> SGVDDDMACHKIPVEADFLYAYSTAPGYYSWRNSKDGSWFIQSLCAMLKQYADKLEFM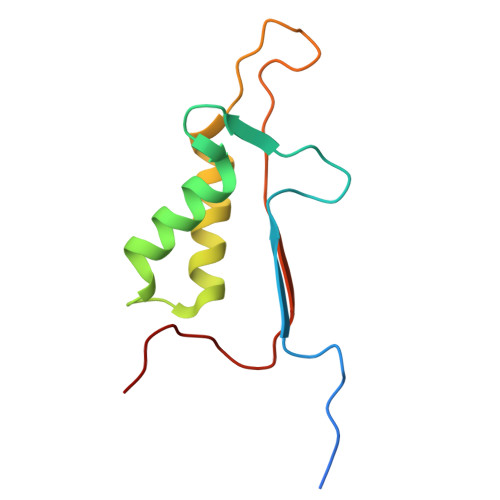HILTRVNRKVADEFEDFSFDATFHAKKQIPCIVSMLTKELYFYHH> KEQLFQSNMERKELHNTVMDLRGNIKVMCRFRPLNEAEILRGDKFIPKFKGEETVVIQGKPYVFDRVLPPNTTQEQVYNACAKQIVKDVLEGYNGTIFAYGQTSSGKTHTMEGKLHDPQLMGIIPRIAHDIFDHIYSMDENLEFAIKVSYFEIYLDKIRDLLDVSKTNLAVHEDKNRVPYVKGCTERFVSSPE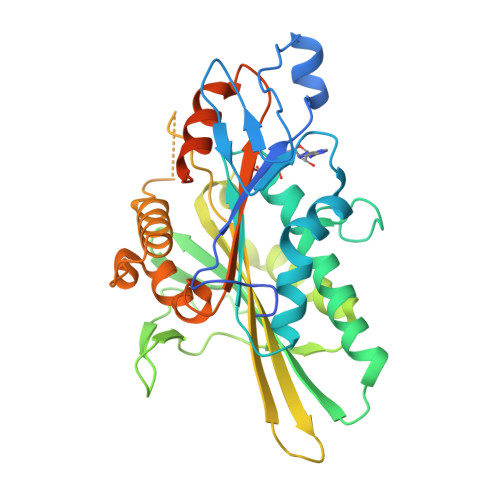EVMDVIDEGKSNRHVAVTNMNEHSSRSHSIFLINIKQENVETEKKLSGKLYLVDLAGSEKVSKTGAEGAVLDEAKNINKSLSALGNVISALAEGTTHVPYRDSKMTRILQDSLGGNCRTTIVICCSPSVFNEAETKSTLMFAASVNSCKMTKAKRNRYLNNSVANSSTQSNNSGSFDK>MRMSDGAAPKANGSEASGQDLVPTAVEQAVPIQPVAGAALAAPAAGQINQIDPWIFQNFVQCPLGEFSISPRNTPGEILFDLALGPGLNPYLAHLSAMYTGWVGNMEVQLVLAGNAFTAGKVVVALVPPYFPKGSLTTAQITCFPHVMCDVRTLEPIQLPLLDVRRVLWHATQDQEESMRLVCMLYTPLRTNSPGDESFVVSGRLLSKPAADFNFVYLTPPIERTIYRMVDLPVLQPRLCTHARWPAPIYGLLVDPSLPSNPQWQNGRVHVDGTLLGTTPVSGSWVSCFAAEAAYEFQSGIGEVATFTLIEQDGSAYVPGDRAAPLGYPDFSGQLEIEVQTETTKKGEKLKVTTFEMILGPT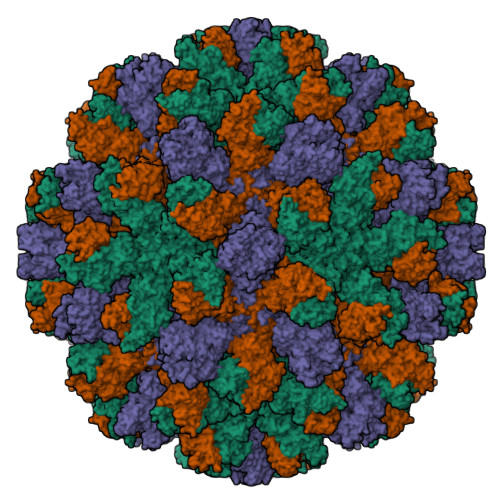TNVDQVPYQGRVYASLTAAASLDLVDGRVRAVPRSVYGFQDVVPEYNDGLLVPLAPPIGPFLPGEVLLRFRTYMRQIDSTDAAAEAIDCALPQEFVSWFASNAFTVQSEALLLRYRNTLTGQLLFECKLYSEGYIALSYSGSGPLTFPTDGFFEVVSWVPRLYQLASVGSLATGRTLKQ[3x]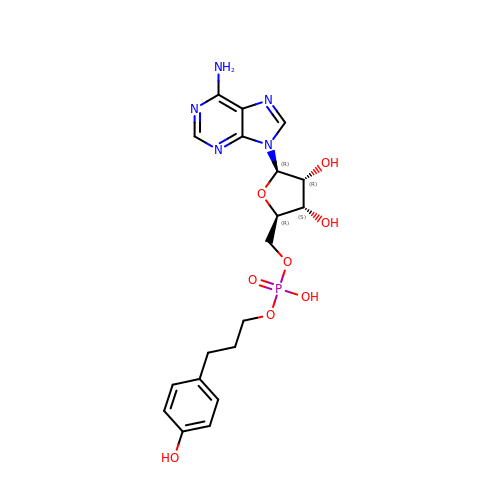5'-O-{(S)-hydroxy[3-(4-hydroxyphenyl)propoxy]phosphoryl}adenosine | C19 H24 N5 O8 P | AWKHKUUJFJBBRQ-NVQRDWNXSA-N> TELTLKPGTLTLAQLRAIHAAPVRLQLDASAAPAIDASVACVEQIIAEDRTAYGINTGFGLLASTRIASHDLENLQRSLVLSHAAGIGAPLDDDLVRLIMVLKINSLSRGFSGIRRKVIDALIALVNAEVYPHIPLKGSVGASGALAPLAHMSLVLLGEGKARYKGQ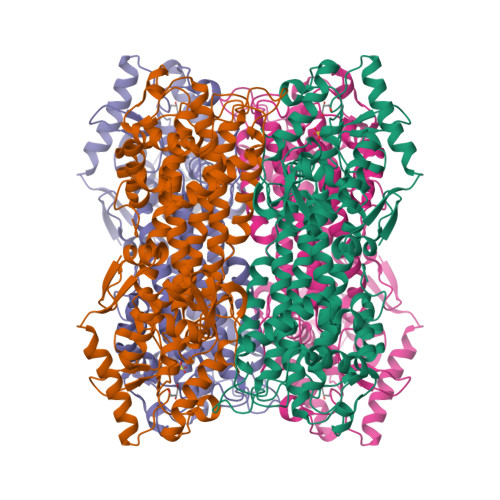WLSATEALAVAGLEPLTLAAKEGLALLNGTQASTAYALRGLFYAEDLYAAAIACGGLSVEAVLGSRSPFDARIHEARGQRGQIDTAACFRDLLGDSSEVSLSHKNADKVQDPYSLRCQPQVMGACLTQLRQAAEVLGIEANAVSDNPLVFAAEGDVISGGNFHAEPVAMAADNLALAIAEIGSLSERRISLMMDKHMSQLPPFLVENGGVNSGFMIAQVTAAALASENKALSHPHSVDSLPTSANQEDHVSMAPAAGKRLWEMAENTRGVLAIEWLGACQGLDLRKGLKTSAKLEKARQALRSEVAHYDRDRFFAPDIEKAVELLAKGSLTGLLPAGVLPSL>[2x]SATAIATLLRNHKELKQRQGLFQAKQTDFFRYKRFVRALHSEEYANKSARQPEIYPTIPSNKIEDQLKSREIFIQLIKAQMVIPVKK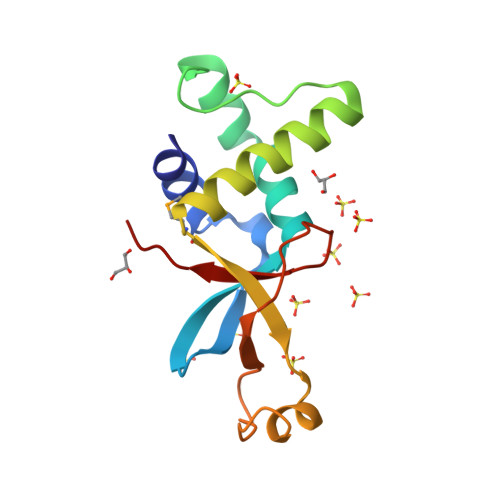LHSQECKEHGLKPSKDFPHLIVSNKAQLEADEYFVWNYNPR>[2x]HGIRMTRISREMMKELLSVYFIMGSNNTKADPVTVVQKALK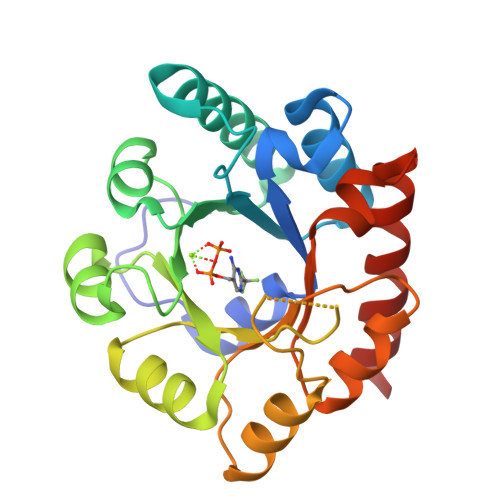GGATLYQFREKGGDALTGEARIKFAEKAQAACREAGVPFIVNDDVELALNLKADGIHIGQEDANAKEVRAAIGDMILGVAAHTMSEVKQAEEDGADYVGLGPIYPTETKKDTRAVQGVSLIEAVRRQGISIPIVGIGGITIDNAAPVIQAGADGVSMISAISQAEDPESAARKFREEIQTYKTGR> VEFVKICGVKTMDELRLVERYADATGVVVN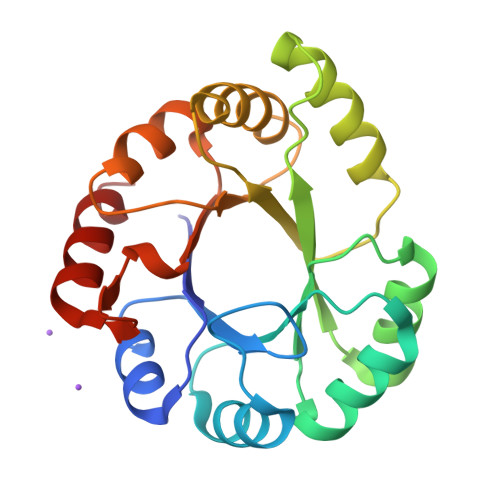SRSKRKVPLKTAAELIEMAEIPIYLVSTMKTFPEWANAVEKTGAEYIQVHSDMHPKAVNRLKDEYGVSVMKAFMVPRESDDPAEDAERLLELIGQYEVDKILLDTGVGSGRRHDYRVSAIIAKEYPIVLAGGLTPENVGEAIRWVKPAGVDVSSGVERNGVKDRVLIEAFMAVVRNG> TAPPEKPRRGWW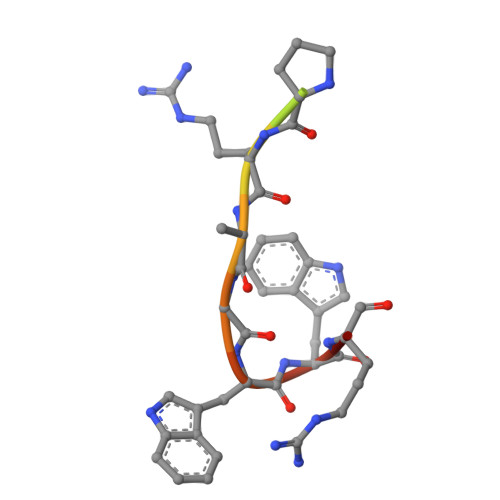RR> MASMTG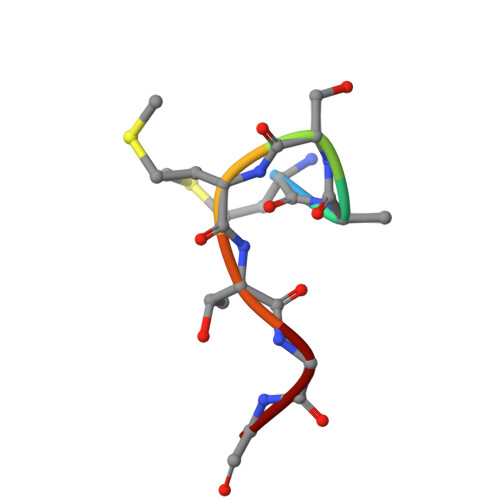G> TFPTYKCPETFDAWYCLNDA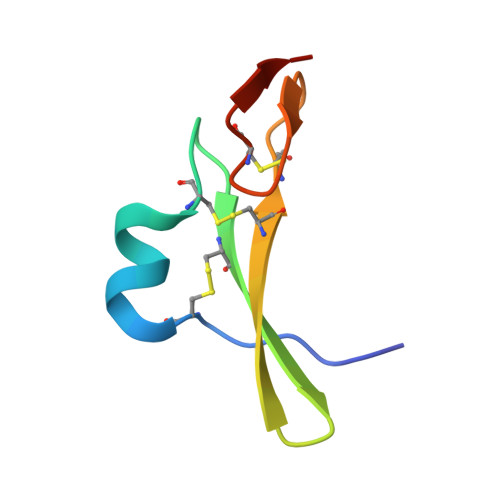HCFAVKIADLPVYSCECAIGFMGQRCEYKEID> SPSVEACGYSDRIMQITRGDSTISSDDVANAVVGYGVWPHYLTPQDATAINKPTQPDTSSNRFYTLESKHWNGSSKGWWWKLPDALKDMGIFGENMYYHFLGRSGYTVHVQCNA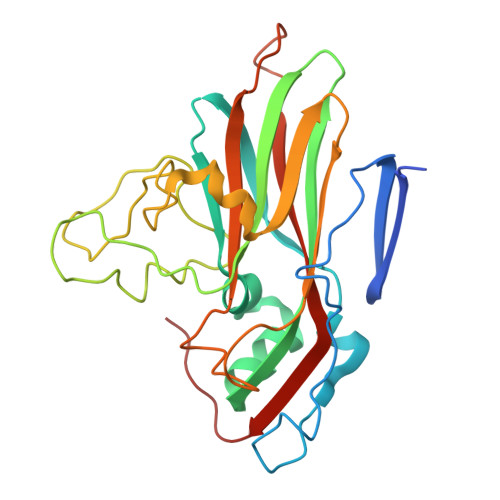SKFHQGTLLVAMIPEHQLASAKHGSVTAGYKLTHPGEAGRDVSQERDASLRQPSDDSWLNFDGTLLGNLLIFPHQFINLRSNNSATLIVPYVNAVPMDSMLRHNNWCLVIIPISPLRSETTSSNIVPITVSISPMCAEFSGARAKNIKQ> GSHMATYYYALGSQKFLLEEEPFEEVLKERRRDYGEKNKEIDFWQVIQPAFLNAPELAEAKAK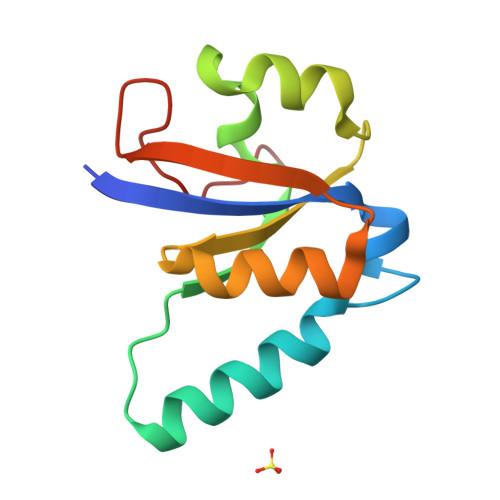APEKNVAIVSTNKSFIVWVKLRLEYVLTGEFEAPSDAIPDPLASLD> MAMHPRKDWYELTRATNWTPSYVTEEQLFPERMSGHMGIPLEKWESYDEPYKTSYPEYVSIQREKDAGAYSVKAALERAKIYENSDPGWISTLKSHYGAIAVGEYAAVTGEGRMARFSKAPGNRNMATFGM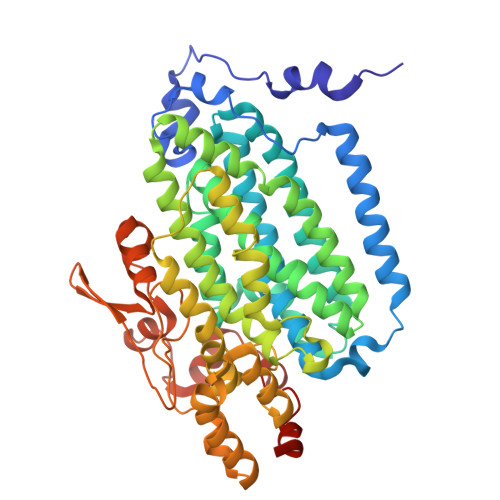MDELRHGQLQLFFPHEYCKKDRQFDWAWRAYHSNEWAAIAAKHFFDDIITGRDAISVAIMLTFSFETGFTNMQFLGLAADAAEAGDYTFANLISSIQTDESRHAQQGGPALQLLIENGKREEAQKKVDMAIWRAWRLFAVLTGPVMDYYTPLEDRSQSFKEFMYEWIIGQFERSLIDLGLDKPWYWDLFLKDIDELHHSYHMGVWYWRTTAWWNPAAGVTPEERDWLEEKYPGWNKRWGRCWDVITENVLNDRMDLVSPETLPSVCNMSQIPLVGVPGDDWNIEVFSLEHNGRLYHFGSEVDRWVFQQDPVQYQNHMNIVDRFLAGQIQPMTLEGALKYMGFQSIEEMGKDAHDFAWADKCKPAMKKSA>GSHMLIAEALELIAEALFAIALALLAIAKKDKELAKKAVELAEKVYKEAEELYKKAKKKGDLIAAALALIAQALAAIALALAAIALKDKELAKKAYKLAEEVYKKAEKLYEEAKKKGDLIAAALALIAQALALIALALAAIALGDKEKLKEVIEKAKEVYKKAEELYKEAEKKGDLIAAALALIAQALALIAIALAAIALGDEETLKEVKEKAKEVYEKAKKVAEEAEKKGDLIAAALALIAQALALIAIALAAIALGDEEELKKVIEEAKKVYEEAKKIYEEAKKKGDLIAAALALIAQALALIAIALAAIALGDEETLEEARKEAEEVKKEAEELAKEAEQK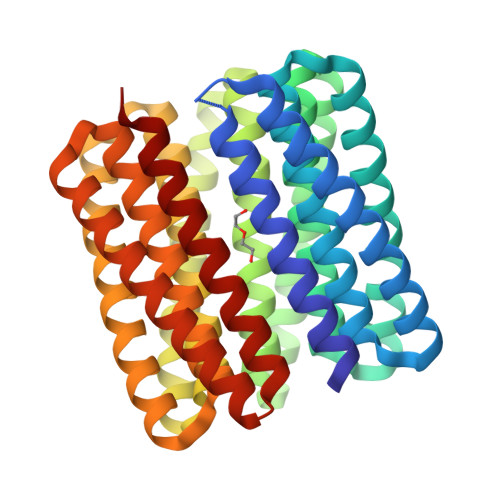GNEIAAALAEIAIALAEIAIALVEIAKK[2x]>ADLNWMSEQNAKLAALLNEAELSEKPIEPVRGHIEGGIAQAYAIQQINVQRQLAAGRRVTGRKIGLTSAAVQKQLGVDQPDFGTLFDSMAVNDGEEIAWSRTLQPKCEAEVALVIERDLDHENITLIDLIGATAYALPAIEVVGSRIANWDINILDTVADNASAGLYVLGHTPVKLEGLDLRLAGMVMERAGQQVSLGVGAACLGHPLNAALWLARTLVKQGTPLKSGDVVLSGALGPLVAANPGDVFEARIQGLGSVRACFSPAS[5x];>AAMKISRIAQRLDEAAVSGKATPQLTGDDAVTVREAAEIQRLLIAHRIERGARQVGLKMGFTSRAKMAQMGVSDLIWGRLTSDMWVEEGGEIDLAHYVHPRVEPEICYLLGKRLEGNVTPLEALAAVEAVAPAMEIIDSRYRDFKFSLPDVIADNASSSG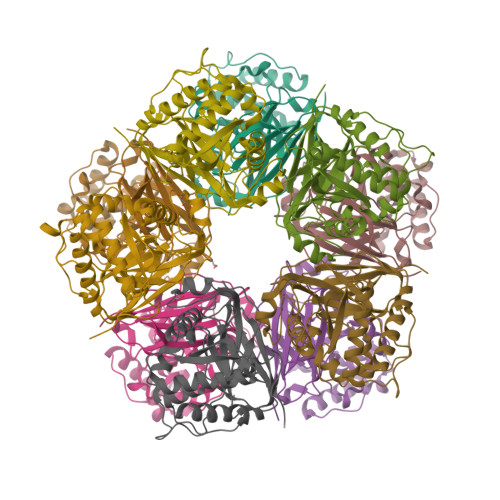FVVGAWHKPETDVSNLGMVMSFDGRAVELGTSAAILGSPIRALVAAARLAAQQGEALEAGSLILAGAATAAVALRPGISVRCEVQNLGSLSFSTTGER[5x]>[8x]MRGSHHHHHHGMASLNRESSNRAKIPEIKIASRKIPNNAALKFVKDMKIGWNLGNTFDAAFENPSFDDELLYETAWCGVKTTKQMIDTVKKAGFNTIRIPVSWHNHVTGSNFTISKRWLDRVQQVVDY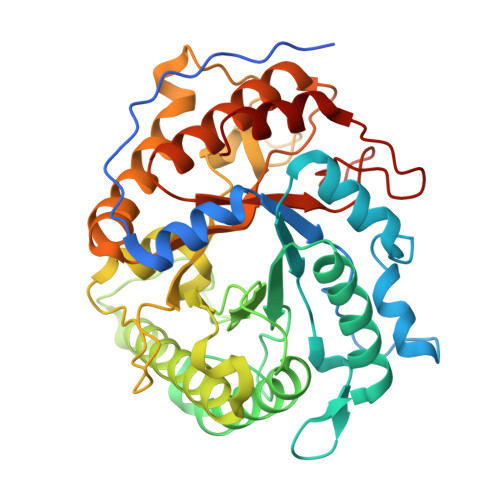AMKNKMYVIINIHHDIMPGYYYPNSQHLQTSIKYVKSIWTQVATRFKNYNDHLIFEAVNEPRLTGSRFEWWLDMNNPECRDAVEAINKLNQVFVDTVRSTGGNNVSRYLMVPGYAAAPEYVLIDEFKIPKDSSKYKNRIIISVHAYRPYNFALQAPNESGSVSEWSVNSEESRRDIDYFMDKLYDKFVSKGIPVVIGEFGARDKNGNLQSRVEFAAYYVRAARARGITCCWWDNNAFYGNGENFGLLDRKTLKWVYPEIVSAMMKYAR> CCGTCG;> GAACGACACCG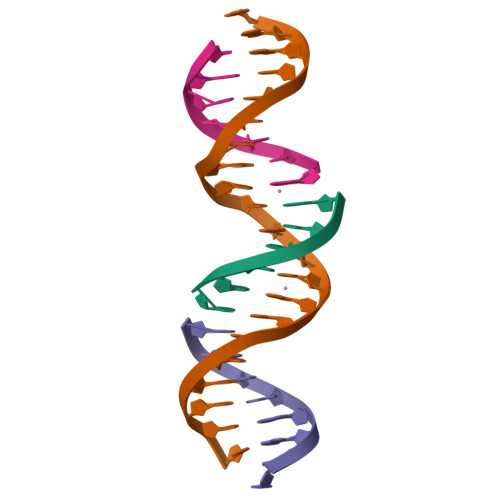ACGGGGACTC;> TCGAGTCC;> GTGTCGT TMEM16 scramblases dissipate the plasma membrane lipid asymmetry to activate multiple eukaryotic cellular pathways. The TMEM16 superfamily is comprised of Cl- channels and dual function scramblases/non-selective ion channels. Our results show afTMEM16 thins the membrane to enable scrambling and that an open hydrophilic pathway is not a structural requirement to allow rapid transbilayer movement of lipids. Scrambling by the TMEM16’s is modulated by two signals, binding of Ca2+ facilitates opening of the groove while the properties of the membrane determine whether the scramblase can thin the membrane enough to enable lipid flipping.

To improve the quality of the density of the lipids near the pathway, we carried out symmetry expansion and additional rounds of 3D classification, which yielded one class with an additional four resolved lipids, for a total of 32 resolved lipids, 16 in each monomer. The observed lipids define the nearly continuous interfaces of the scramblase with the inner and outer membrane leaflets near the dimer interface (lipids D1-D9) and illustrate how the poses adopted by individual lipids result in the profound remodeling of the membrane induced by afTMEM16 near the lipid pathway (lipids P1-P7). The C18/Ca2+ structure reveals how the scramblase reorients the lipids that approach the open scrambling pathway. The downward slope of the OL starts at D5, a well-defined PG lipid, and progresses towards the open groove as P1 and P2 adopt distorted poses with their headgroups becoming increasingly tilted. The IL bends upwards and P5-P7 become increasingly tilted as their heads climb around the intracellular portions of TM3 and TM4, coordinated by the hydrophilic side chains of T341, K345 and T334. At the pathway, P3 is sandwiched between TM4 and TM6 near the constriction formed by T325 and Y432 and its headgroup points towards the extracellular side, such that it is contiguous to other OL lipids. Notably, P3 and P4 are oriented with their heads facing the outside of the groove. The distance between the phosphate atoms of the heads of P3 and P4 in the OL and IL is <22 Å, showing that the hydrocarbon core of the membrane is thinned by ~50% at the open pathway. One unexpected feature of our structure is that the extracellular vestibule of the groove does not directly interact with the membrane and no lipids could be resolved there, as they cross the open groove at the T325 and Y432 constriction. The wide intracellular vestibule is embedded in the nanodisc membrane and, at the open pathway, the P3 and P4 lipids have opposite orientations, suggesting scrambling might occur in the groove region comprised between them.

> MAFNPAPKAVQENHHVDYVIRFNYGDIDTPEAIKKFEVLLLELSEVGLQTEVRQGDENSLFVFVRAASKKKLKRAVYQSRVRDWLYGVRNTEPEPASSAKPQSEAERLLVIYHLITVPKAEGGAGITPRHGEWKNVDAIFPLHDEETNRQCMREWSKKTFLSTEDLDRIRNTFGEHVGFYFAFLQSYFRFLMFPAAFGFSCWLLLGSFSIIYTVVNCLWCIVFIEYWKRQEEDLSCRWQTKGVSAVHEKRAEFKPEKEIRDESTGEVRGVFPATKRMYRQLLQVPFALLAAVALGAIIATCFAIEIFISEVYNGPLKGYLVFIPTILVSALIPTMSAVLLTVATKLNDYENYETQDAYKVALTQKIFVVNFITSYLPIILTAFVYVPFASRIVPYLDVFHLTVRPFVSKEHAIKARTEFSINPDRLRKQVIYFTVTAQIVGFALETIVPFVKQRVFREYKEYTKKQHAKAEPGNGAGEKKTVSLGDDEDEARFLTRVRNEAELEDYDVTDDLREMCIQFGYLALFSPVWPLVPVSFLINNWVELRSDFFKICVECKRPWPQRADTIGPWLDSLGFLSWVGSITSSALVYMFSNGHEGPNGEPTTIRCWALLLTIFFSEHLYLIVRYAVRSALAKLEPPNTRRERIERFMMRKRYLDTVLSAESDDDADEVKGVVSSIPPSEITRESLEQDARDWSKQGTDPTERFWMRQRGWKESAEVGLSLITKAKGDETKKQQ1-(4-tert-butylphenyl)-2-[(1S,2R,5S,8R,8aR)-1,2,8-trihydroxyoctahydroindolizin-5-yl]ethanone | C20 H29 N O4 | 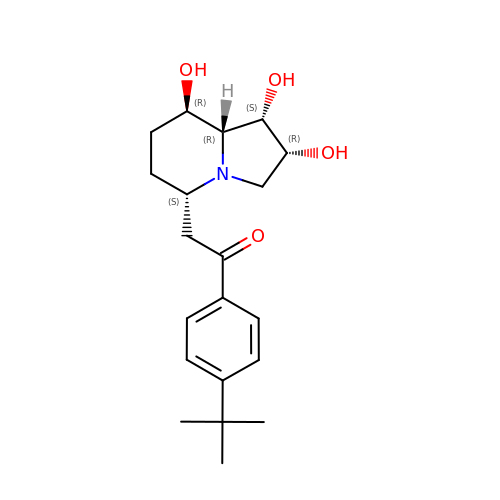PKZGDTMZYSPKOW-ZPKKHLQPSA-N>[2x]MKPKVVLTHWVHPEIIELLSASADVIPNTTRETLPRSEVIARAKDADALMAFMPDSIDSAFLEECPKLRVIGAALKGYDNFDVNACTRHGVWLTIVPDLLTIPTAELTIGLLLGLTRHMLEGDRQIRSGHFQGWRPTLYGSGLTGKTLGIIGMGAVGR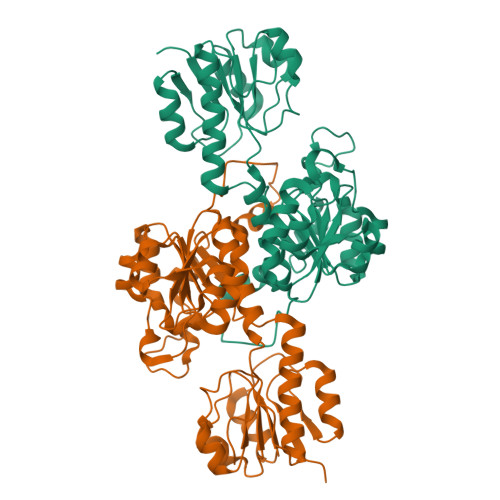AIAQRLAGFEMNLLYCDPIPLNAEQEKAWHVQRVTLDELLEKCDYVVPMVPMAAETLHLIDATALAKMKTGSYLINACRGSVVDENAVIAALASGKLAGYAADVFEMEEWIRADRPQAIPKALLDNTAQTFFTPHLGSAVKEVRLEIERQAAMNIIQALAGEKPMGAINQPYPGVKAA> AKYLELEEGGVIM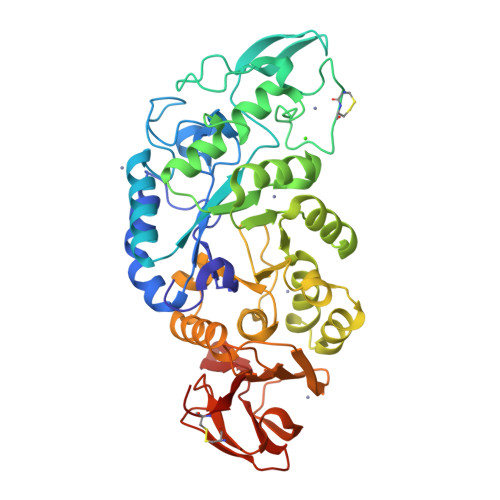QAFYWDVPGGGIWWDHIRSKIPEWYEAGISAIWLPPPSKGMSGGYSMGYDPYDYFDLGEYYQKGTVETRFGSKEELVRLIQTAHAYGIKVIADVVINHRAGGDLEWNPFVGDYTWTDFSKVASGKYTANYLDFHPNELHCCDEGTFGGFPDICHHKEWDQYWLWKSNESYAAYLRSIGFDGWRFDYVKGYGAWVVRDWLNWWGGWAVGEYWDTNVDALLSWAYESGAKVFDFPLYYKMDEAFDNNNIPALVYALQNGQTVVSRDPFKAVTFVANHDTDIIWNKYPAYAFILTYEGQPVIFYRDFEEWLNKDKLINLIWIHDHLAGGSTTIVYYDNDELIFVRNGDSRRPGLITYINLSPNWVGRWVYVPKFAGACIHEYTGNLGGWVDKRVDSSGWVYLEAPPHDPANGYYGYSVWSYCGVG> GAASGAKSLFSTAFSESLAAEISSVSRDELMEAIQKQEEINFRL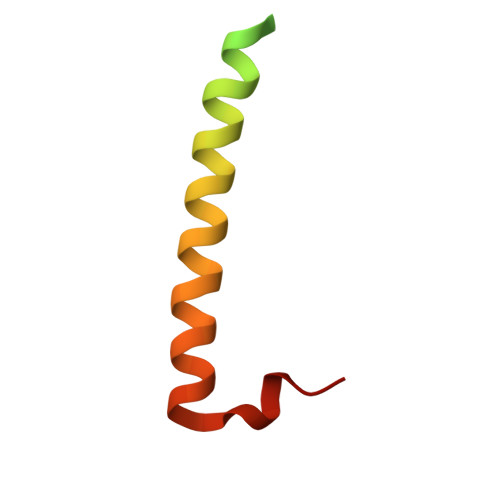QDYIDRIIVAIMETNPSILEVK> GAMASGKVVKFSYMWTINNFSFCREEMGEVIKSSTFSSGANDKLKWCLRVNPKGLDEESKDYLSLYLLLVSCPKSEVRAKFKFSILNAKGEETKAMESQRAYRFVQGKDW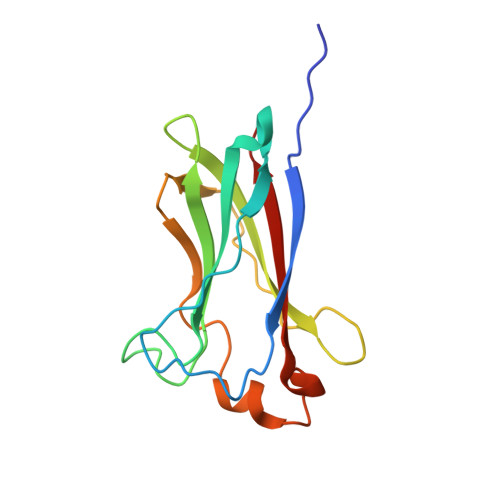GFKKFIRRDFLLDEANGLLPDDKLTLFCEVSVVQD>[4x]MSDAHVLKSRLEWGEPAFTILDVRDRSTYNDGHIMGAMAMPIEDLVDRASSSLEKSRDIYVYGAGDEQTSQAVNLLRSAGFEHVSELK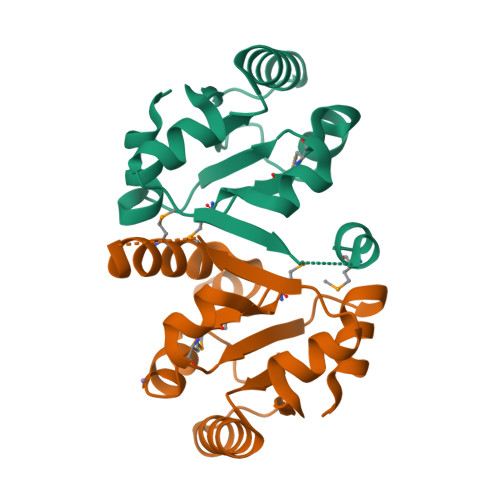GGLAAWKAIGGPTEGIIESRTPAGADDYNVVSRMQNHLENQKKEVLEHHHHHH> GDGPYLQILEQPKQRGFRFRYVCEGPSHGGLPGASSEKNKKSYPQVKICNYVGPAKVIVQLVTN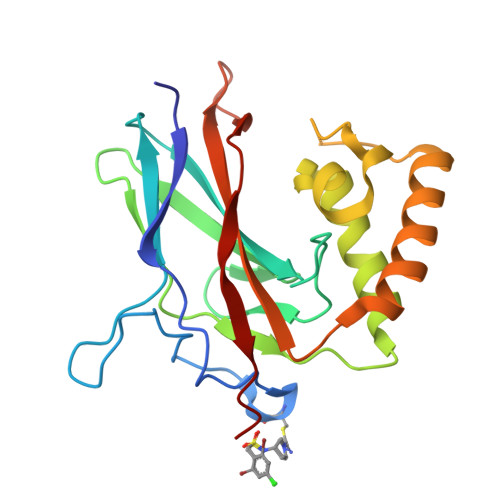GKNIHLHAHSLVGKHCEDGICTVTAGPKDMVVGFANLGILHVTKKKVFETLEARMTEACIRGYNPGLLVHPDLAYLQAEGGGDRQLGDREKELIRQAALQQTKEMDLSVVRLMFTAFLPDSTGSFTRRLEPVVSDAIYDSKAP> NHTNVKFLFDRSRLLNVIKVLEKDAVFPRPFPTATGTQQDDGYFCLLTPRPTVASRPATRFGLYVSPSDSGVLANTSLDFNFYSLACFTYFRSDLEVTVVSLEPDLEFAVGWFPSGSEYQASSFVYDQLHVPYHFTGRTPRAFASKGGKVSFVLPWNSVSSVLPVRWGGASKLSSATRGLPAHADWGTIYAFIPRPNEKKSTAVKHVAVYIRYKNARAWCPSMLPFRSYK;> VLCAYVEDPTKSDPPSSSTDQPTTTFTAIDRWYTGRLNSWTKAVKTFSFQAVPLPGAFLSRQGGLNGGAFTATLHRHFLMKCGWQVQVQCNLTQFHQGALLVAMVPETTLDVKPDGKAKSLQELNEEQWVEMSDDYRTGKNMPFQSLGTYYRPPNWTWGPNFINPYQVTVFPHQILNARTSTSVDINVPYIGETPTQSSETQNSWTLLVMVLVPLDYKEGATTDPEITFSVRPTSPYFNGLRNRYT;> GPIPTAPRENSLMFLSTTPDDTVPAYGNVRTPPVNYLPGEITDLLQLARIPTLMAFGRVPEPEPASDAYVPYVAVPTQFDDKPLISFPITLSDPVYQNTLVGAISSNFANYRGCIQITLTFCGPMMARGKFLLSYSPPNGTQPQTLSEAMQCTYSIWDIGLNSSWTFVIPYISPSDYRETRAITNSVYSADGWFSLHKLTKITLPP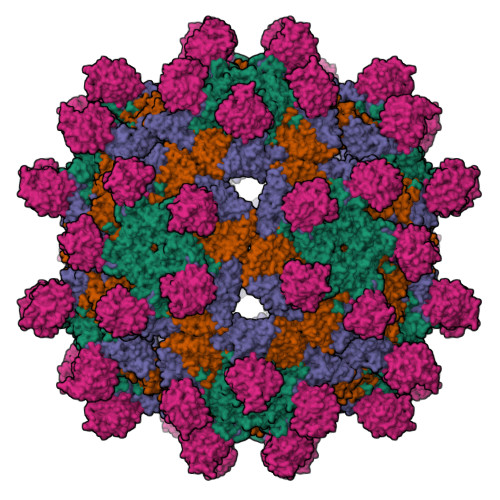DCPQSPCILFFASAGEDYTLRLPVDCNPSYVF;> SMACYGGFDLYFILDKSGSVLHHWNEIYYFVEQLAHKFISPQLRMSFIVFSTRGTTLMKLTEDREQIRQGLEELQKVLPGGDTYMHEGFERASEQIYYENRQGYRTASVIIALTDGELHEDLFFYSEREANRSRDLGAIVYAVGVKDFNETQLARIADSKDHVFPVNDGFQALQGIIHSILKKSC> XADEIAKAQVARPGGDTIFGKIIRKEIPAKIIFEDDRCLAFHDIS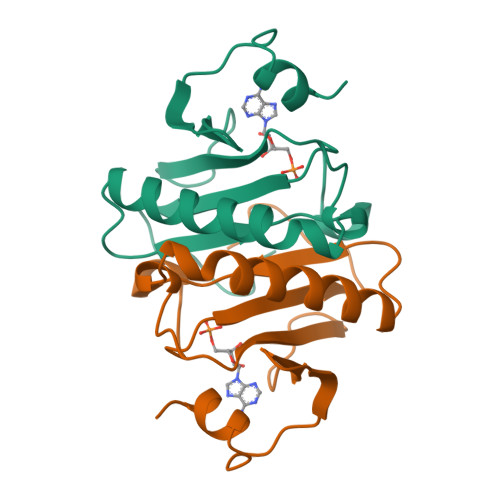PQAPTHFLVIPKKHISQISVAEDDDESLLGHLMIVGKKCAADLGLNKGYRMVVNEGSDGGQSVYHVHLHVLGGRQMHWPPG>MLLNVAGPLGTPVPMEKFGKILAIGAYTGIVEVYPIAKAWQEIGNDVTTLHVTFEPMVILKEELEKAVTRHIVEPVPLNPNQDFLANMKNVSQRLKEKVRE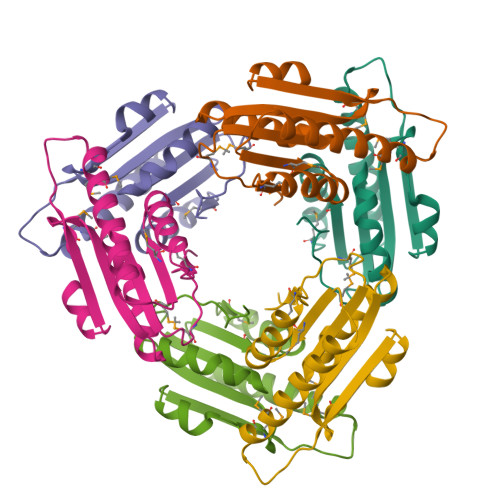LLESEDWDLVFMVGPVGDQKQVFEVVKEYGVPMLEHHHHHH[6x]Moiramide B | C25 H31 N3 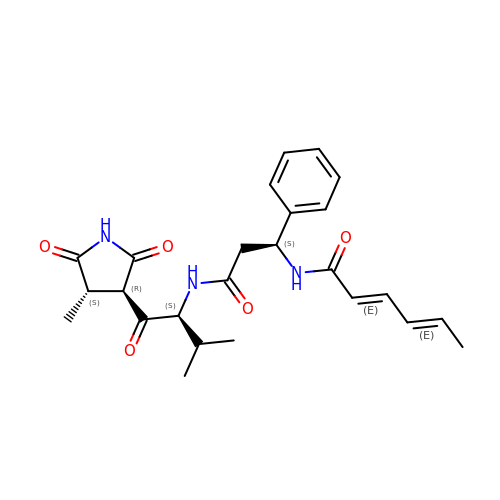O5 | WMLLJSBRSSYYPT-PQUJRENYSA-N>MAGVRLSLLKSIQRSIKPHATAKSCSGLLNSHARAFTCGNLLDGPKASPSMISFSSNIRLHNDAKPFNYLGHSSYARAFSSKSDDFGSIVASGVTGSGDGNGNGNDWVEKAKDVLQTSVDAVTETAKKTKDVSDEMIPHVQQFLDSNPYLKDVIVPVSLTMTGTLFAWVVMPRILRRFHTYAMQSSAKLLPVGFSNEDVPYEKSFWGALEDPARYLVTFIAFAQIAAMVAPTTAIAQYFSPTVKGAVILSLVWFLYRWKTNVITRMLSAKSFGGLDREKVLTLDKVSSVGLFAIGLMASAEACGVAVQSILTVGGVGGVATAFAARDILGNVLSGLSMQFS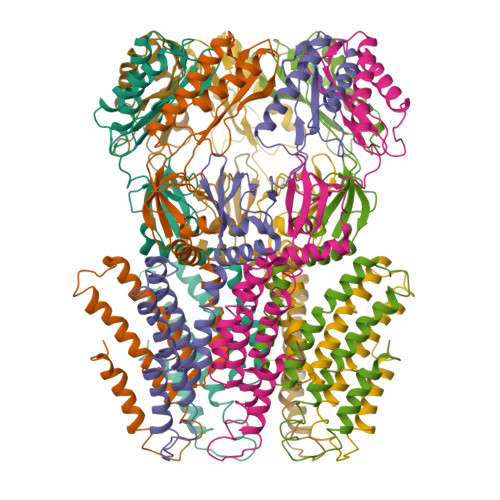RPFSMGDTIKAGSVEGQVIEMGLTTTSLLNAEKFPVLVPNSLFSSQVIVNKSRAQWRAIASKIPLQIDDLDMIPQISNEIKEMLRSNTKVFLGKEAPHCYLSRVEKSFAELTIGCNLIRMGKEELYNTQQEVLLEAVKIIKKHGVSLGTTWDNSTL[7x]>MKSVSFSNNAELYEYIKDKKNDVEIVACIITNLLGTYFKCFFYVKEITLNKLESGFSFDASSIKLCSDTEVSDFFIKVDHSTCYLEECDGKNILNIMCDIKRYNGFDYYKCPRTILKKTCEFVKNEGIADKVCIGNELEFFIFDKVNYSLDEYNTYLKVYDRESFSCKNDLSSIYGNHVVNKVEPHKDHFNNPNNEYLINDDSKKVKKKSGYFTTDPYDTSNIIKLRICRALNDMNINVQRYHHEVSTSQHEISLKYFDALTNADFLLITKQIIKTTVSSFNRTATFMPKPLVNDNGNGLHCNISLWKNNKNIFYHNDPSTFFLSKESFYFMYGIVKHAKALQAFCNATMNSYKRLVPGFETCQKLFYSFGSRSAVIRLSLINYSNPSEKRIEFRLPDCANSPHLVMAAIILAGYDGIKSKEQPLVPFESKDNHFYISSIFSKYVQHPENFNILTHALEGYESLHTINESPEFKNFFKCEEPQGISFSLVESLDALEKDHAFLTVNNIFTEEMIQEYIKFKREEIDAYNKY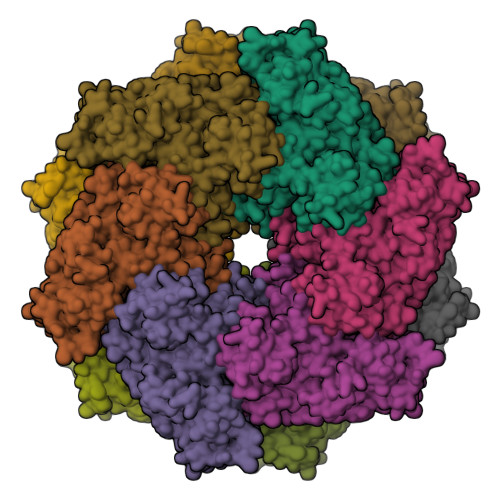VNAYDYHLYYEC[12x]Glyceraldehyde-3-phosphate dehydrogenase (GAPDH) is a highly conserved enzyme involved in the ubiquitous process of glycolysis and presents a loop (residues 208–215 of Escherichia coli GAPDH) in two alternative conformations (I and II). In the presence of inorganic phosphate (Pi), GAPDH catalyzes the conversion of D-glyceraldehyde-3-phosphate (G3P) to 1,3-diphosphoglycerate (BPG), accompanying the reduction of NAD+ to NADH. All the structures reported in this paper have four subunits: O, P, Q, and R. Each subunit contained two domains: the C-terminal catalytic domain and the N-terminal NAD+-binding domain. Two anion recognition sites, “Ps” and “Pi”, bind the C3 phosphate of G3P and inorganic phosphate, respectively.

In order to see whether Cys150 and His177 could affect enzyme activity and structure, we obtained mutants H177A, C150S, C150A, C150A+H177A, and C150S, whose structures were the most similar to that of the wild type. The enzymatic activity of wild-type EcGAPDH1 was 3.84 × 104 times higher than that of C150S and 8.13 × 103 times higher than that of H177A. These results indicate that C150 and H177 are essential for EcGAPDH1 activity.

>HHHHHHSSGLVPRGSHMASMSKVGINGFGRIGRLVLRRLLEVKSNIDVVAINDLTSPKILAYLLKHDSNYGPFPWSVDFTEDSLIVDGKSIAVYAEKEAKNIPWKAKGAEIIVECTGFYTSAEKSQAHLDAGAKKVLISAPAGEMKTIVYNVNDDTLDGNDTIVSVASSTTNCLAPMAKALHDSFGIEVGTMTTIHAYTGTQSLVDGPRGKDLRASRAAAENIIPHTTGAAKAIGLVIPELSGKLKGHAQRVPVKTGSVTELVSILGKKVTAEEVNNALKQATTNNESFGYTDEEIVSSDIIGSHFGSVFDATQTEITAVGDLQLVKTVAWYDNEYGFVTQLIRTLEKFAKL[4x]>GGAGCUC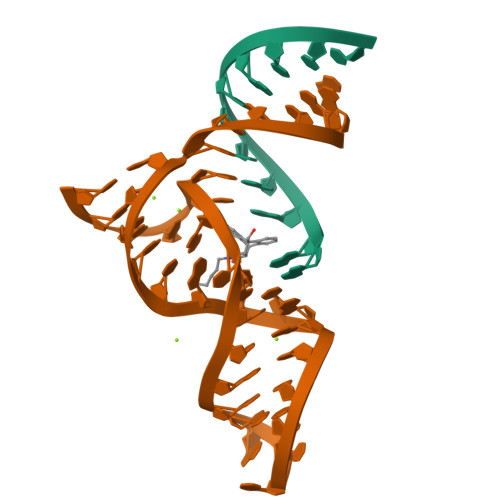GCCC[2x];>GGGCGAGGCCGUGCCAGCUCUUCGGAGCAAUACUCGGC[2x]> GSGSGSGSGSSKFSNITIKNFRNFEKVNINLDNKNVIFGMNDIGKTNFLYALRFLLDKEIRKFGFNKSDYHKHDTSKKIEIILTLDLSNYEKDEDTKKLISVVKGARTSANADVFYIALESKYDDKELYGNIILKWGSELDNLIDIPGRGNINALDNVFKVIYINPLVDLDKLFAQNKKYIFEESQGNESDEGILNNIKSLTDQVNQQIGEMTIIKGFQQEITSEYRSLKKEEVSIELKSEMAIKGFFSDIIPYIKKDGDSNYYPTSGDGRRKMLSYSIYNYLAKKKYEDKIVIYLIEEPEISLHRSMQIALSKQLFEQSTYKYFFLSTHSPELLYEMDNTRLI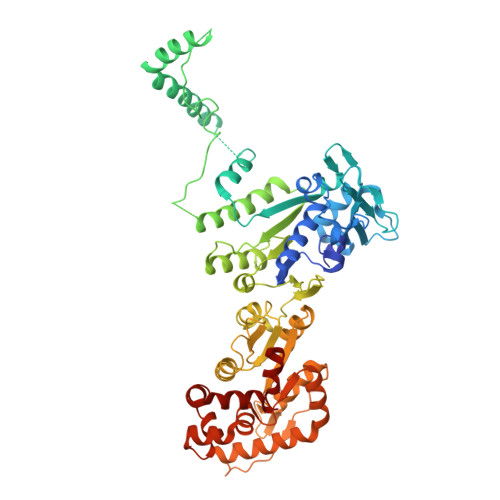RVHSTEKVVCSSHMYNVEEAYGSVKKKLNKALSSALFAERVLLIEGPSEKILFEKVLDEVEPEYELNGGFLLEVGGTYFNHYVCTLNDLGITHIIKTDNDLKSKKGKKGVYELLGLNRCLNLLGRENLDEITIDIPEDIKGKKKKERLNERKKEIFKQYKNEVGEFLGERIYLSEIDLENDLYSAIGESMKRIFENEDPVHYLQKSKLFNMVELVNNLSTKDCFDVFEHEKFACLKELVGSDRG>RWAPIPASLMENSLGPFPQHVQQIQSDAAQNYTIFYSISGPGVDKEPFNLFYIEKDTGDIFCTRSIDREKYEQFALYGYATTADGYAPEYPLPLIIKIEDDNDNAPYFEHRVTIFTVPENCRSGTSVGKVTATDLDEPDTLHTRLKYKILQQIPDHPKHFSIHPDTGVITTTTPFLDREKCDTYQLIMEVRDMGGQPFGLFNTGTITISLEDENDNPPSFTETSYVTEVEENRIDVEILRMKVQDQDLPNTPHSKAVYKILQGNENGNFIISTDPNTNEGVLCVVKPLNYEVNRQVILQVGVINEAQFSKAASSQTPTMCTTTVTVKIIDSDEGPE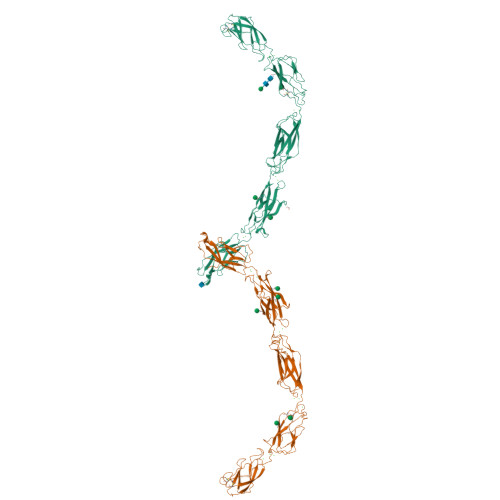CHPPVKVIQSQDGFPAGQELLGYKALDPEISSGEGLRYQKLGDEDNWFEINQHTGDLRTLKVLDRESKFVKNNQYNISVVAVDAVGRSCTGTLVVHLDDYNDHAPQIDKEVTICQNNEDFAVLKPVDPDGPENGPPFQFFLDNSASKNWNIEEKDGKTAILRQRQNLDYNYYSVPIQIKDRHGLVATHMLTVRVCDCSTPSECRMKHHHHHH[2x]> PISPIETVPVKLKPGMDGPKVKQWPLTEEKIK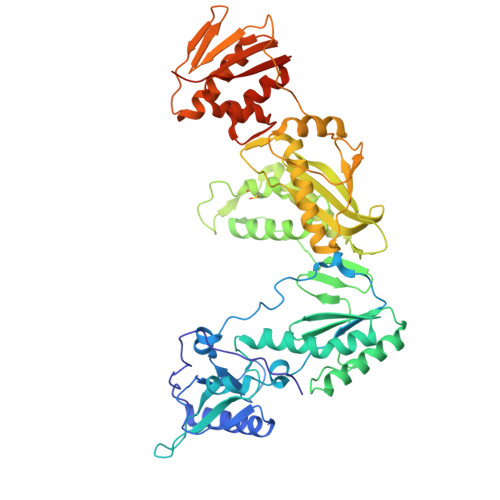ALVEICTEMEKEGKISKIGPENPYNTPVFAIKKKDSTKWRKLVDFRELNKRTQDFWEVQLGIPHPAGLKKKKSATVLDVGDAYFSVPLDEDFRKYTAFTIPSINNETPGIRYQYNVLPQGWKGSPAIFQSSMTKILEPFRKQNPDIVIYQYMDDLYVGSDLEIGQHRTKIEELRQHLLRWGLTTPDKKHQKEPPFLWMGYELHPDKWTVQPIVLPEKDSWTVNDIQKLVGKLNWASQIYPGIKVRQLCKLLRGTKALTEVIPLTEEAELELAENREILKEPVHGVYYDPSKDLIAEIQKQGQGQWTYQIYQEPFKNLKTGKYARMRGAHTNDVKQLTEAVQKITTESIVIWGKTPKFKLPIQKETWETWWTEYWQATWIPEWEFVNTPPLVKLWYQLEKEPIVGAETFYVDGAANRETKLGKAGYVTNRGRQKVVTLTDTTNQKTELQAIYLALQDSGLEVNIVTDSQYALGIIQAQPDQSESELVNQIIEQLIKKEKVYLAWVPAHKGIGGNEQVDKLVSAGIRKVL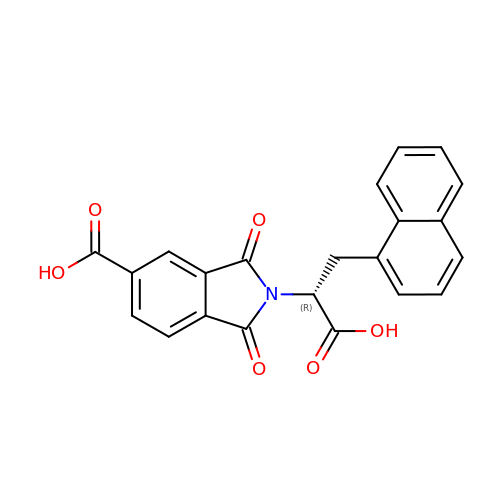2-[(1R)-1-carboxy-2-naphthalen-1-ylethyl]-1,3-dioxo-2,3-dihydro-1H-isoindole-5-carboxylic acid | C22 H15 N O6 | CZNPWASYMRBJCX-GOSISDBHSA-N(2R,6S,13aR,14aR,16aS)-6-{[(cyclopentyloxy)carbonyl]amino}-14a-[(cyclopropylsulfonyl)carbamoyl]-5,16-dioxooctadecahydrocyclopropa[e]pyrrolo[1,2-a][1,4]diazacyclopentadecin-2-yl 3,4-dihydroisoquinoline-2(1H)-carboxylate | C37 H51 N5 O9 S | 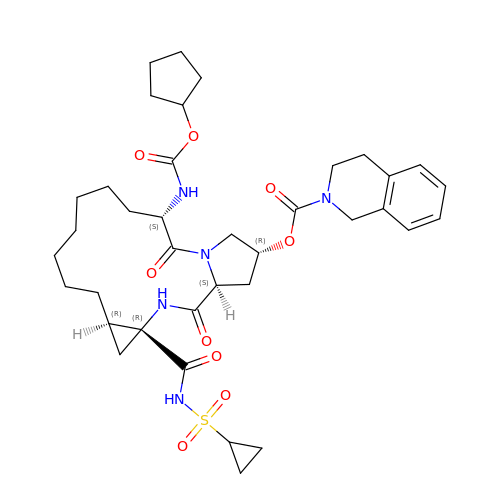VQZYSHWAKCNHJX-IVYVMHIUSA-N2-[benzyl(methyl)amino]ethyl methyl 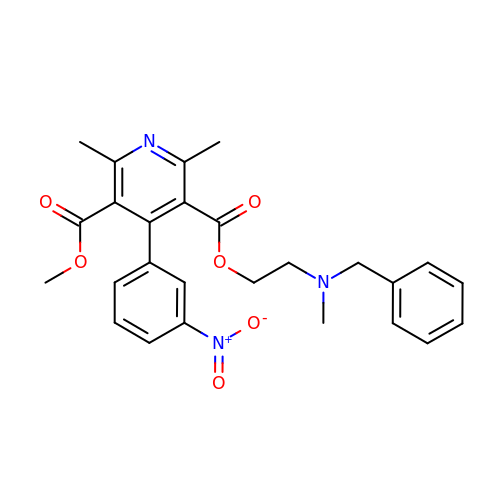2,6-dimethyl-4-(3-nitrophenyl)pyridine-3,5-dicarboxylate | C26 H27 N3 O6 | GROZWIBBDLLXKU-UHFFFAOYSA-N>[24x]GDTKEQRILRYVQQNAKPGDPQSVLEAIDTYCTQKEWAMNVGD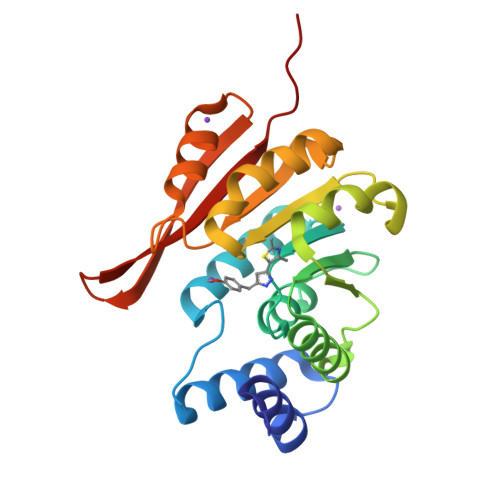AKGQIMDAVIREYSPSLVLELGAYCGYSAVRMARLLQPGARLLTMEINPDCAAITQQMLNFAGLQDKVTILNGASQDLIPQLKKKYDVDTLDMVFLDHWKDRYLPDTLLLEECGLLRKGTVLLADNVIVPGTPDFLAYVRGSSSFECTHYSSYLEYMKVVDGLEKAIYQGPSSD(2E)-3-(3-chloro-5-{2-[2-(2,4-dioxo-3,4-dihydropyrimidin-1(2H)-yl)ethoxy]-4-[2-(morpholin-4-yl)ethoxy]phenoxy}phenyl)prop-2-enenitrile 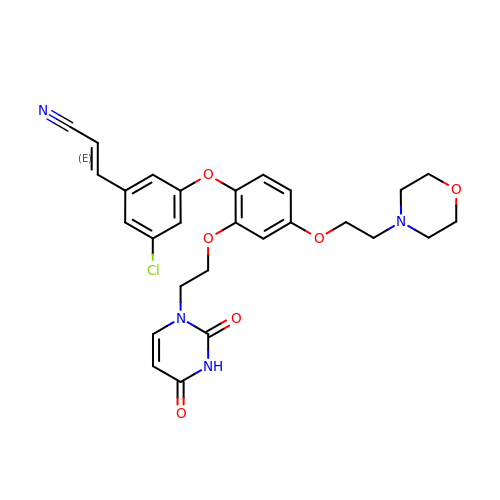| C27 H27 Cl N4 O6 | DTELLJHPYARPQX-OWOJBTEDSA-N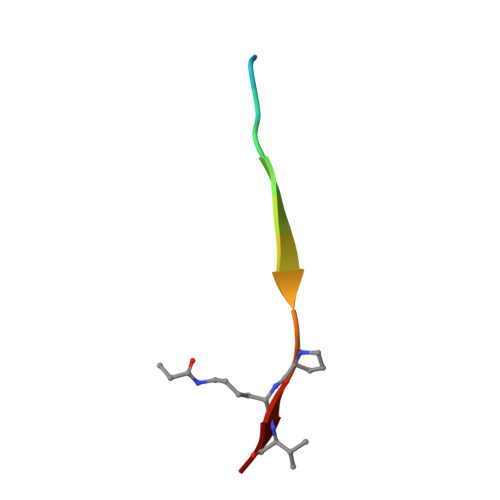> XKLRPVAMVRPXVR> MPFVNKQFNYKDPVNGVDIAYIKIPNAGQMQPVKAFKIHNKIWVIPERDTFTNPEEGDLNPPPEAKQVPVSYYDSTYLSTDNEKDNYLKGVTKLFERIYSTDLGRMLLTSIVRGIPFWGGSTIDTELKVIDTNCINVIQPDGSYRSEELNLVIIGPSADIIQFECKSFGHEVLNLTRNGYGSTQYIRFSPDFTFGFEESLEVDTNPLLGAGKFATDPAVTLAHELIHAGHRLYGIAINPNRVFKVNTNAYYEMSGLEVSFEELRTFGGHDAKFIDSLQENEFRLYYYNKFKDIASTLNKAKSIVGTTASLQYMKNVFKEKYLLSEDTSGKFSVDKLKFDKLYKMLTEIYTEDNFVKFFKVL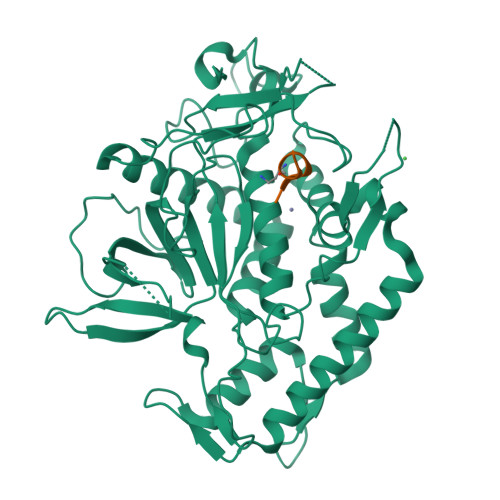NRKTYLNFDKAVFKINIVPKVNYTIYDGFNLRNTNLAANFNGQNTEINNMNFTKLK;> XRWTAMLG> MRIVEVYSHLNGLEYIQVHLPHIWEEIQEIIVSIDAEACRTKESKEKTKQGQILYSPV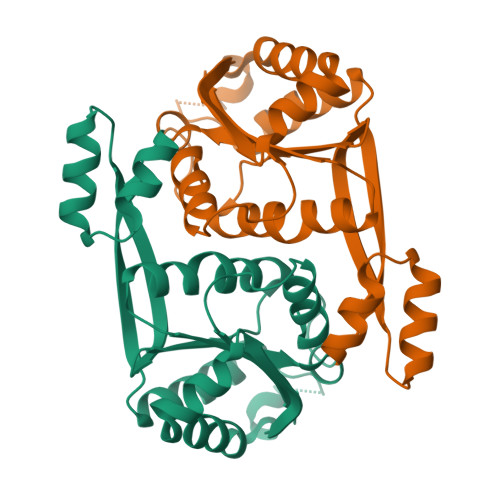ALNEAFKEKLEAKGWKESRTNYYVTADPKLIRETLSLEPEEQKKVIEAAGKEALKSYNQTDFVKDRVAIEVQFGKYSFVAYDLFVKHMAFYVSDKIDVGVEILPMKELSKEMSSGISYYEGELYNVIRQGRGVPAVPLVLIGIAP As a proof-of-concept, five peptidoglycan hydrolases from the Acinetobacter baumannii proteome (PHAb7-PHAb11) were identified using PlyF307 lysin-derived peptide as a template. To understand the catalytic mechanism and thermal stability of these peptidoglycan hydrolases, we attempted to decipher their structures and eventually obtained the crystal structures of PHAb8, PHAb10, and PHAb11 by X-ray crystallography. Despite their lower amino acid sequence similarity, PHAb8, PHAb10, and PHAb11 superimposed well with T4 lysozyme, especially in their Glu-Asp-Thr catalytic triad regions, suggesting that PHAb8, PHAb10, and PHAb11 may be phage-originated. All these observations together indicated that PHAb8, PHAb10, and PHAb11 were highly evolutionarily related to T4 lysozyme and might share similar catalytic mechanisms of action.

We solved the crystal structures of PHAb8, PHAb10, and PHAb11 and unveiled that hyper-thermostable PHAb10 underwent a unique folding-refolding thermodynamic scheme mediated by a dimer-monomer transition, while thermosensitive PHAb8 formed a monomer. Results showed that PHAb8 was a monomer, while PHAb10 and PHAb11 formed an asymmetric dimer. Interestingly, PHAb8 showed high topological similarity to monomeric PHAb10 and PHAb11, with the typical catalytic triad (Glu-Asp-Thr) located at the coil region. In contrast, PHAb7, PHAb8, and PHAb9 completely lost their activity after treatment at 70°C for 1 hr. Our results showed that PHAb8, PHAb10, and PHAb11 were denatured with transition temperatures of 41.4°C, 53.7°C, and 59.9°C, respectively. Interestingly, signs of aggregation were only observed in PHAb8 but not in PHAb10 and PHAb11, indicating that PHAb10 and PHAb11 underwent structural refolding without precipitation during heat treatment.

> MSVDNAEQIAQAYSWLRAMSGGKLTQEQVTAGDSIIAMNGLKTFAQVIGYKMSDAVTGFRDISENGYKLIKSFEGFEPKAYQDTGGVWTIGYGTIKYPNGTRVKKGDMCTMAEAEEWLKNDCAWVDACLDKYLKFQPTQNQFDALASFVYNVGETAFSKSTMLKSLNAGNFAGAANQFDKWVYDNGKLIKGLVNRRAAEKKLFLS> MNHKVHHHHHHIEGRHMTISVPGHGTLGAPDGAAAPGGEAAELPPLVPEPGDAGQPFPLTPTQQALWVGRADAVDLGDIGCYGYFEWERPELDLARYRRAWERLVAHHPGLRTVVRPDGTQHVLERPGPVPITVEDLRQDPDAVRRLEESRAERGHRALDPGTWPMFDLRVVLLSGRVRVQLGIDLQLMDASSLFLNLFSDLVTLYDDPDAALASQKLAFRDFARWLEEDVRGGARWRADWAYWQERLDGLPPAPDLPAARYGAQGPGKFERCMVRCPAEEFALLRERALAHGLTETELLVGAFAEVLRGWSSDPAFTLNVPVFQRFDVPGIEDVIGDYTNPILLEARPEGRTVAERIVALAARLRADTRHASVNGVEVLRELARRRGLAAAAMPVVVTSLLGLPSAARSITEFGTEVHSITQTPQVSLDFQIRPEDGELRLVWDHRSGAFAPGVVEGAFEAFLDLVGRMLADEPGHGVWEAPFADMRSRRDRAVWNETNDTAEPVPAVLLQERFFAQARRTPDAEAVVASGLRLTYDELARHAYRIGNTLRERGVRPGDLVGVVMEKGWEQYAAVYGILAAGGAYLPIDAASPRGRVARLLESAGAGIVLTQSRLRDELDLPAGTTVLRADTDFETASTAPLTPVQGPDDPAYVIYTSGSTGEPKGVVVAHRGVANLVRDVRRRFAVTPADRLLALSGLHFDASVYDVFGPLACGATVV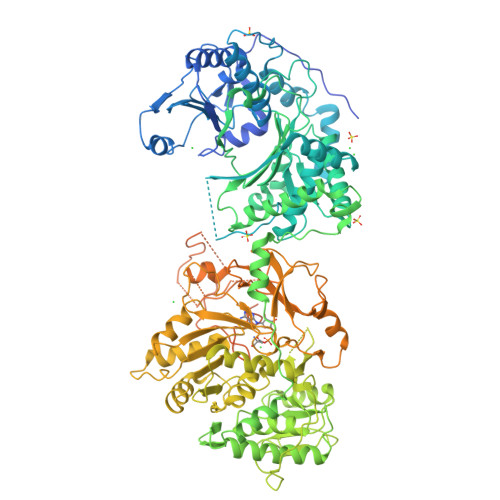VPPPFRRAEPDVWAELVRDERVTFWNSVPVLLELLVGEAESRDDRPLATLRLAVVSGDWIPLDLPGRARAQAPGLRVVGSGGPTETICWSLFHPIDAVDPQWTSIPYGKPIANQRYYIVDRDLRPRPTWARGEMAVASPLGLALGYLNDPERTAAKFVTLPGTGERAYLTGDFGRLLPDGGIEILGREDFQVKVAGQRIELGEIEALLHRADGVRAAVVTAPRSSADVVRLQAFVVPETGARLSADALREHLSAELPAAMVPAAIRLLPELPLTANGKVDRLALARLAAAPEEAPEPEARTDYAPRTDVGLLAELVAACVAELLGLDEVPTTGNFFRLGGDALSGTRLASRLQDLLGAPVPIRTVFGNPVLGDLASAIAGDPAAGPQAIRVARLLHTLEEPDEKPGEKPDAEPAGEPDAGSRTSAWSHPQFEK>HHHHHIEGRHMAGPDRAELAELVRRLSVVHGRVTLSSGREADYYVDLRRATLHHRASALIGRLMRELTADWDYSVVGGLTLGADPVATAIMHAPGRPIDAFVVRKSAKAHGMQRLIEGSEVTGQRVLVVEDTSTTGNSALTAVHAVQDVGGEVVGVATVVDRATGAAEAIEAEG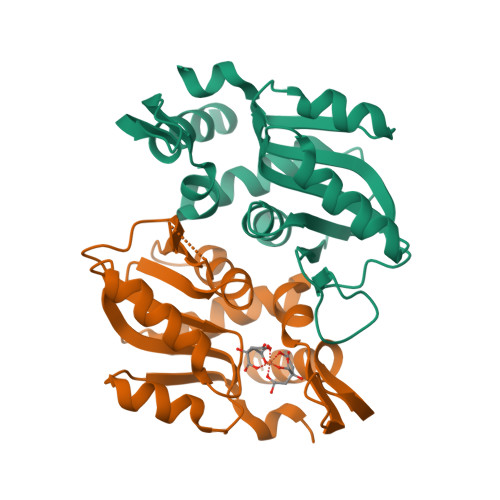LRYRSVLGLADLGLD[4x]> MGHHHHHHHHENLYFQGSGLSTKSQPVIQATLPVIAERIPHITPVFYGDMLQARPDLLDGMFSRSAQRDGTQARALAGSIAIFAQWILQHPNTFPEEMLSRVANKHASLGLQPDEYDTVYKYLFGAIAKDLGDAATPDIVEAWTEVYWLLARALINLERKLYAQQANNIVRAKFKLVKRTQVTKDVVDMVFEPADNTAMTPGKAGQYISIYARTSDGLLQPRQFTLLPSEETQRRIAIKLDPHGEMTTIFQNQEVGALLDISNPYGDMTLETLETDPNSPLVLICAGIGVTPVLAFVEKLAAQKSEREVMIIASSRSLAEAPLRGELLERAKELKKAKVLYGTTQEKDGDFVGRIDVSTLDIPANASVFLCGPLKFMQEMR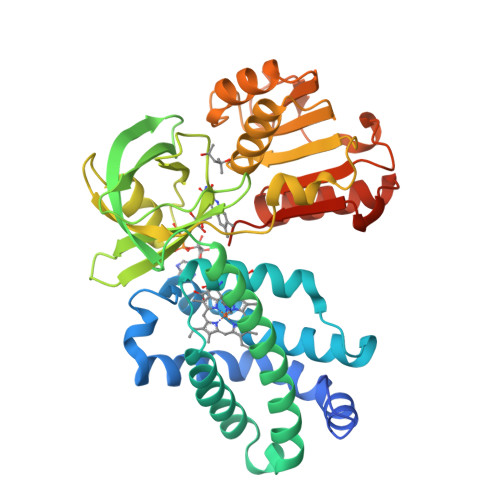SHLVEAGIAKHKIFYEIFGTDQWMLHDQNRSE> MKRKKNFIWIAILLVGVVMVMYYAVKKHNDINQKTDKNY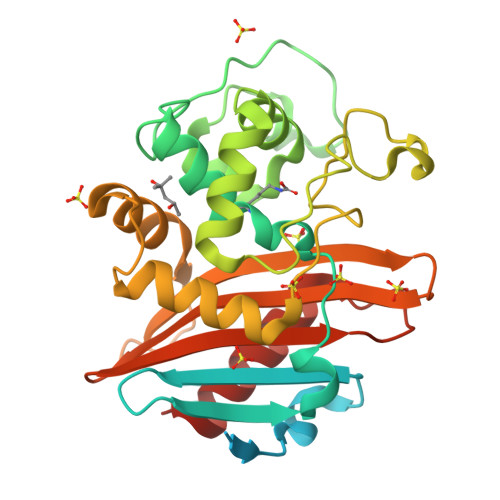IKSELNKSKIKNNDKNKKESVNIVDYSDCFEGISGGAIFCNTKNKEYNIYNKELIETRRSPCSTFKIVSTLIGLEKGVINSKESVMGYDGTDYPNKNWNKNLSLEEAFKESCVWYYKKLINKVDAKSVQNILDDLKYGNCDISEWEGDLKNGKGHLNGFWLESSLQISPKEQVQTMAKIFEGDTNFKKEHINILRDIMAIDVNDANINVYGKTGTGFDEKNKRVDAWFVGMLEREGDTYYFAIKSDDSNKEITGPKVKEIAINIIKKYYSVRE> FKIETTPESRYLAQIGDSVSLTCSTTGCESPFFSWRTQIDSPLNGKVTNEGTTSTLTMNPVSFGNEHSYLCTA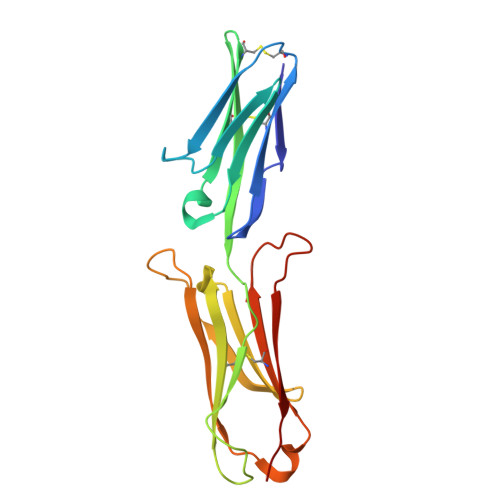TCESRKLEKGIQVEIYSFPKDPEIHLSGPLEAGKPITVKCSVADVYPFDRLEIDLLKGDHLMKSQEFLEDADRKSLETKSLEVTFTPVIEDIGKVLVCRAKLHIDEMDSVPTVRQAVKELQVY> MSAIERISKAAHLIDMCDIIREGNPSLRTVAEEVTFPLSDQEIILGEKMMQFLKHSQDPVMAEKMGLRGGVGLAAPQLDISKRIIAVLVPNIVEEGETPQEAYDLEAIMYNPKIVSHSVQDAALG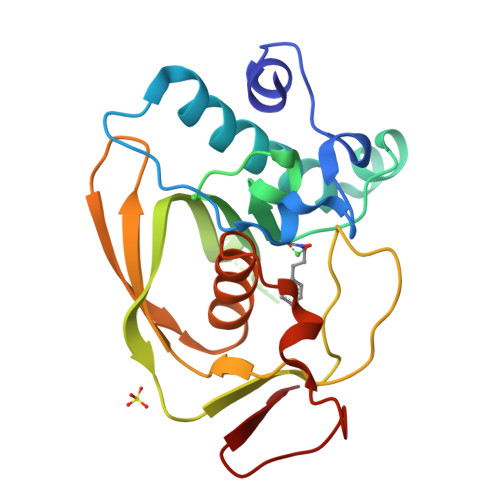EGEGCLSVDRNVPGYVVRHARVTVDYFDKDGEKHRIKLKGYNSIVVQHEIDHINGIMFYDRINEKDPFAVKDGLLILE> IVGEALEYVNIGLSHFLALPLAQRISLIIIIPFIYNIVWQLLYSLRKDRPPLVFYWIPWVGSAVVYGMKPYEFFEECQKKYGDIFSFVLLGRVMTVYLGPKGHEFVFNAKLADVSAEAAYAHLTTPVFGKGVIYDCPNSRLMEQKKFVKGALTKEAFKSYVPLIAEEVYKYFRDSKNFRLNERTTGTIDVMVTQPEMTIFTASRSLLGKEMRAKLDTDFAYLYSDLDKGFTPINFVFPNLPLEHYRKRDHAQKAISGTYMSLIKERRKNNDIQDRDLIDSLMKNSTYKDGVKMTDQEIANLLIGVLMGGQHTSAATSAWILLHLAERPDVQQELYEEQMRVLDGGKKELTYDLLQEMPLLNQTIKETLRMHHPLHSLFRKVMKDMHVPNTSYVIPAGYHVLVSPGYTHLRDEYFPNAHQFNIHRWNNDSASSYSVGEEVDYGFGAISKGVSSPYLPFGGGRHRCIGEHFAYCQLGVLMSIFIRTLKWHYPEGKTVPPPDFTSMVTLPTGPAKIIWEKRNPEQKIGGRH

A common mechanism of resistance among fungal pathogens occurs due to mutations in the enzymatic target of azole drugs, the cytochrome P450 lanosterol 14α-demethylase (denoted as Erg11p or CYP51). Azoles inhibit the demethylase by coordinating to the heme iron in the active site via a heterocyclic nitrogen atom of an imidazole, triazole or tetrazole ring. In the present study, new high-resolution X-ray crystal structures of the ScErg11p6 × His Y140F mutant in complex with ITC, FLC, VCZ and PCZ and the Y140H mutant in complex with FLC and ITC, along with the wild type ScErg11p6 × His in complex with VCZ, provide evidence that disruption of this hydrogen bond network leads to weaker drug binding. We have created and analysed the structure and function of surrogate triazole resistance phenotypes in the yeast S. cerevisiae by creating Y140F/H single site mutations in lanosterol 14α-demethylase that have homologues in numerous species of pathogenic fungi. This study shows how alterations to a water-mediated hydrogen-bonding network, between the drug and target protein, can affect the affinity of the short-tailed triazole drugs FLC and VCZ but not the long-tailed triazoles ITC and PCZ.

The pyrimidine ring of VCZ occupies a similar position to the non-coordinating triazole ring of FLC but projects further into the substrate channel. The 5-fluoro substituent of the pyrimidine ring projects towards Y126 forcing this residue close enough to interact with the heme ring A propionate (2.8 Å; as seen in complexes with the long-tailed azoles PCZ and ITC). The key water molecule (743) is present and forms a similar hydrogen-bonding network with the phenolic hydroxyl of Y140, the heme ring D propionate and the tertiary hydroxyl group of VCZ. An additional hydrogen bond is present between the 5-fluoro substituent and the key water 743 (3.0 Å), which is shifted slightly towards Y140. The water molecule corresponding to water 790 in the FLC structure is not present at this position due to the projection of the pyrimidine ring. However, a water molecule (750) seen in complexes with the long-tailed azoles is also seen here. It forms hydrogen bonds between the pyrimidine nitrogen (N1), the main chain nitrogens of H381 and S382 plus the carbonyl of residue M509 which projects into the binding site cavity. The water-mediated polar interactions between Y140 and the tertiary hydroxyl of FLC and VCZ optimally stabilise the binding of these drugs.> AVADDFQASVMGPLAKINDWGSFKKQLQTLKNNGVYAITTDVWWGYVESAGDNQFDWSYYKTYANAVKEAGLKWVPIISTHKCGGNVGDDCNIPLPSWLSSKGSADEMQFKDESGYANSEALSPLWSGTGKQYDELYASFAENFAGYKSIIPKIYLSGGPSGELRYPSYYPAAGWSYPGRGKFQAYTETAKNAFRTAMNDKYGSLDKINAAWGTKLTSLSQINPPTDGDGFYTNGGYNSAYGKDFLSWYQSVLEKHLGVIGAAAHKNFDSVFGVRIGAKISGLHWQMNNPAMPHGTEQAGGYYDYNRLIQKFKDA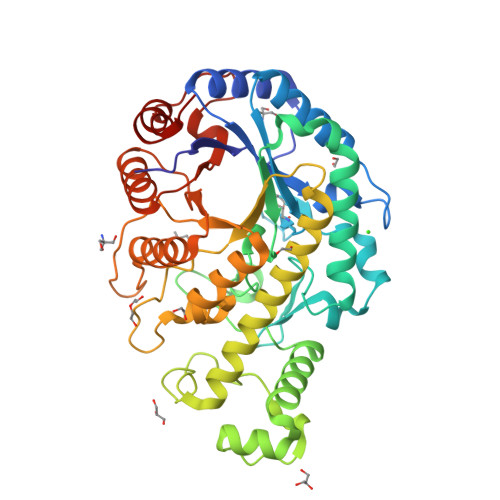DLDLTFTCLEMSDSGTAPNYSLPSTLVDTVSSIANAKGVRLNGENALPTGGSGFQKIEEKITKFGYHGFTLLRINNLVNNDGSPTGELSGFKQYIISKAKPDNN>[2x]DYKDDDDKLAAAQYPVVNTNYGKIRGLRTPLPNEILGPVEQYLGVPYASPPTGERRFQPPEPPSSWTGIRNTTQFAAVCPQHLDERSLLHDMLPIWFTANLDTLMTYVQDQNEDCLYLNIYVPTEDDIHDQNSKKPVMVYIHGGSYMEGTGNMIDGSILASYGNVIVITINYRLGILGFLSTGDQAAKGNYGLLDQIQALRWIEENVGAFGGDPKRVTIFGSGAGASCVSLLTLSHYSEGLFQKAIIQSGTALSSWAVNYQPAKYTRILADKVGCNMLDTTDMVECLRNKNYKELIQQTITPATYHIAFGPVIDGDVIPDDPQILMEQGEFLNYDIMLGVNQGEGLKFVDGIVDNEDGVTPNDFDFSVSNFVDNLYGYPEGKDTLRETIKFMYTDWADKENPETRRKTLVALFTDHQWVAPAV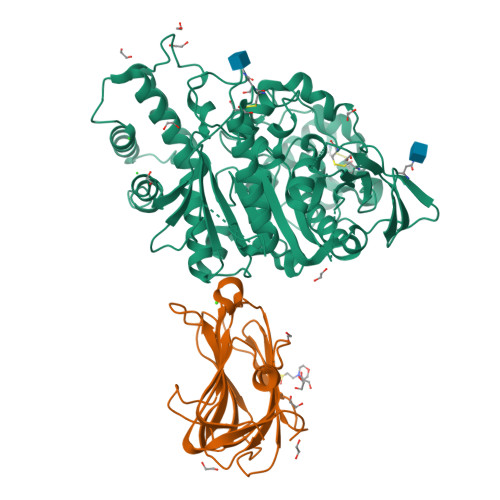ATADLHAQYGSPTYFYAFYHHCQSEMKPSWADSAHGDEVPYVFGIPMIGPTELFSCNFSKNDVMLSAVVMTYWTNFAKTGDPNQPVPQDTKFIHTKPNRFEEVAWSRYNPKDQLYLHIGLKPRVRDHYRATKVAFWLELVPHLHNLNEIFQYVSTTTKVPPPDMT;>GGHAGTTYIFSKGGGQITYKWPPNDRPSTRADRLAIGFSTVQKEAVLVRVDSSSGLGDYLELHIHQGKIGVKFNVGTDDIAIEESNAIINDGKYHVVRFTRSGGNATLQVDSWPVIERYPAGRQLTIFNSQATIIIGGKEQGQPFQGQLSGLYYNGLKVLNMAAENDANIAIVGNVRLV[2x]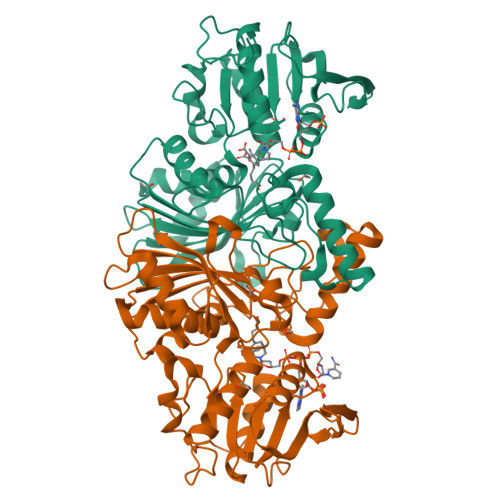>MGYTVAVVGATGAVGAQMIKMLEESTLPIDKIRYLASARSAGKSLKFKDQDITIEETTETAFEGVDIALFSAGSSTSAKYAPYAVKAGVVVVDNTSYFRQNPDVPLVVPEVNAHALDAHNGIIACPNCSTIQMMVALEPVRQKWGLDRIIVSTYQAVSGAGMGAILETQRELREVLNDGVKPCDLHAEILPSGGDKKHYPIAFNALPQIDVFTDNDYTYEEMKMTKETKKIMEDDSIAVSATCVRIPVLSAHSESVYIETKEVAPIEEVKAAIAAFPGAVLEDDVAHQIYPQAINAVGSRDTFVGRIRKDLDAEKGIHMWVVSDNLLKGAAWNSVQIAETLHERGLVRPTAELKFELKLEHHHHHH[2x]(4S,5E,8S,9E,11S,13E,15E,18R)-8-methoxy-9,11-dimethyl-18-[(1Z,4E)-2-methylhexa-1,4-dien-1-yl]-2-oxooxacyclooctadeca-5,9,13,15-tetraen-4-yl 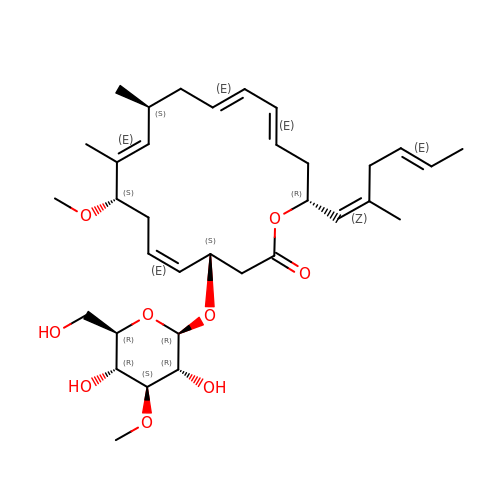3-O-methyl-beta-D-glucopyranoside | C34 H52 O9 | QLNOFWPLTFNJPW-CMAVNLJPSA-N>GSSKEVAELKKQVESAELKNQRLK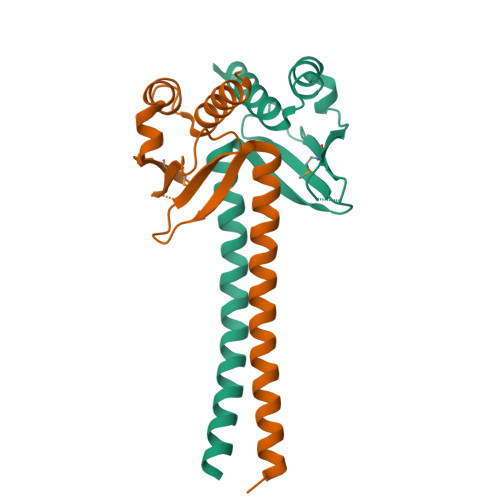EVFQTKIQEFRKACYTLTGYQIDITTENQYRLTSLYAEHPGDCLIFKATSPSGSKMQLLETEFSHTVGELIEVHLRRQDSIPAFLSSLTLELFSRQTVA[2x]mesobiliverdin IX(alpha) | C33 H38 N4 O6 | 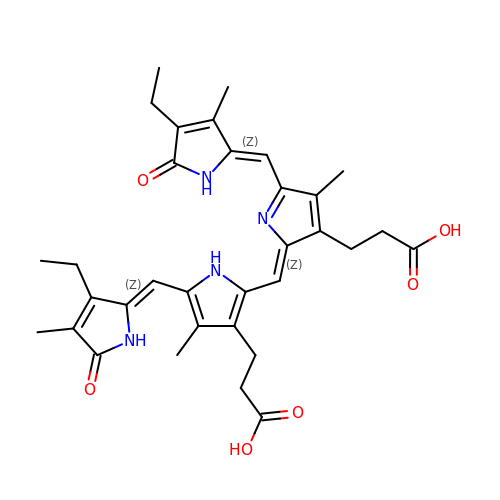CXQHEXWJGZEPFP-BBROENKCSA-N>ANPCCSNPCQNRGECMSTGFDQYKCDCTRTGFYGENCTTPEFLTRIKLLLKPTPNTVHYILTHFKGVWNIVNNIPFLRSLIMKYVLTSRSYLIDSPPTYNVHYGYKSWEAFSNLSYYTRALPPVADDCPTPMGVKGNKELPDSKEVLEKVLLRREFIPDPQGSNMMFAFFAQHFTHQFFKTDHKRGPGFTRGLGHGVDLNHIYGETLDRQHKLRLFKDGKLKYQVIGGEVYPPTVKDTQVEMIYPPHIPENLQFAVGQEVFGLVPGLMMYATIWLREHNRVCDILKQEHPEWGDEQLFQTSRLILIGETIKIVIEDYVQHLSGYHFKLKFDPELLFNQQFQYQNRIASEFNTLYHWHPLLPDTFNIEDQEYSFKQFLYNNSILLEHGLTQFVESFTRQIAGRVA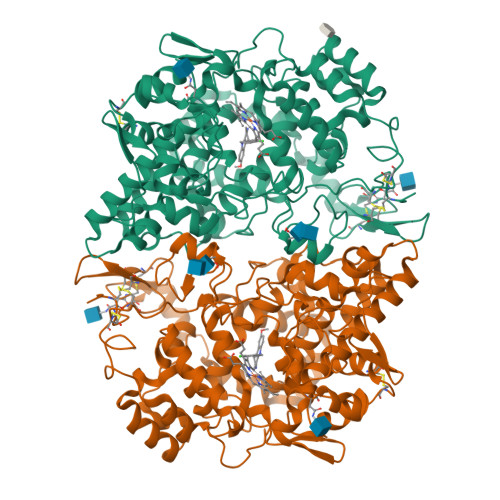GGRNVPIAVQAVAKASIDQSREMKYQSLNEYRKRFSLKPYTSFEELTGEKEMAAELKALYSDIDVMELYPALLVEKPRPDAIFGETMVELGAPFSLKGLMGNPICSPQYWKPSTFGGEVGFKIINTASIQSLICNNVKGCPFTSFNVQDPQPTKTATINASASHSRLDDINPTVLIKRRSTEL[4x]>DKMNSVGEACTDMKREYDQCFNRWFAEKFLKGDSSG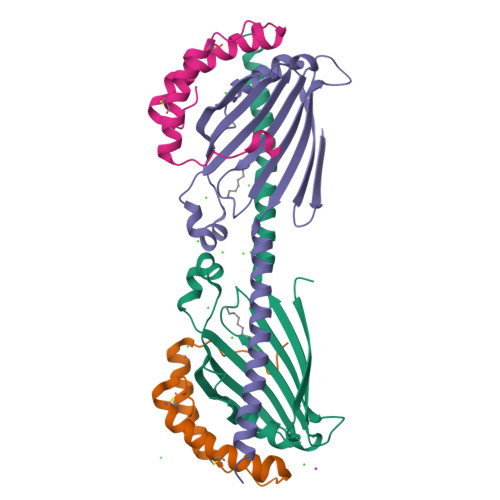DPCTDLFKRYQQCVQKAIKEKEIPIEGLEFMGH[2x];>HHHHHHSDQMVKYFLGQSVLRSSWDQVFAAFWQRYPNPYSKHVLTEDIVHREVTPDQKLLSRRLLTKTNRMPRWAERLFPANVAHSVYVLEDSIVDPQNQTMTTFTWNINHARLMVVEERSVYSVNSDNSGWTEIRREAWVSSSLFGVSRAVQEFGLARFKSNVTKTMKGFEYILAKLQGEA[2x]>GMPQHDKSRLVRIDTGPMINPVAGKPSRPIAGDASFRTVTAFEGGQGKVESGVWESTSGSFQSNTTGYIEYCHIIEGEAR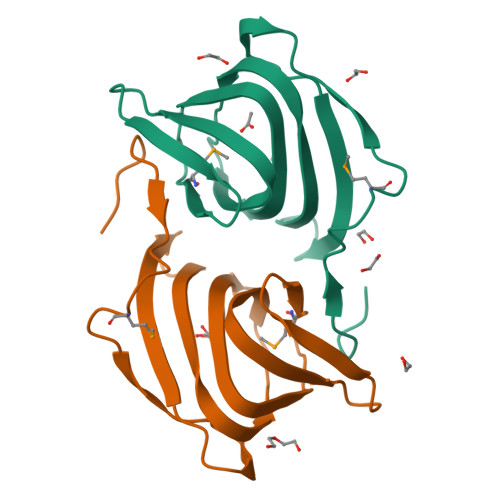LVDPDGTVHAVKAGDAFIMPEGYTGRWEVDRHVKKIYFVTHLA[2x]> GAQVSTQKTGAHETSLSASGNSTIHYTNINYYKDAASNSANRQDFTQDPGKFTEPVKD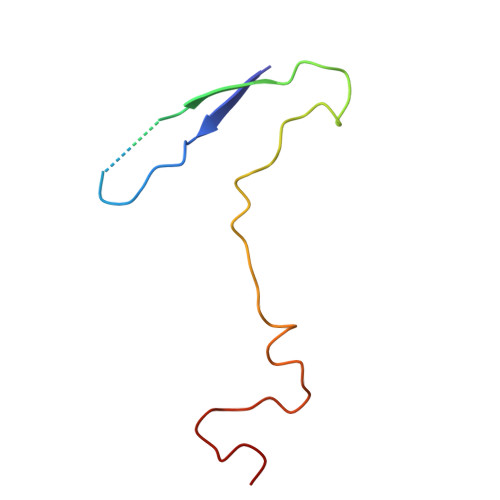IMVKSLPALN> DPTYADYFSAWDKWEKQALPGEERDEAVSRLKECLINNSDELRLDRLNLSSLPDNLPAQITLLNVSYNQLTNLPELPVTLKKLYSASNKLSELPVLPPALESLQVQHNELENLPALPDSLLTMNISYNEIVSLPSLPQALKNLRATRNFLTELPAFSEGNNPVVREYFFDRNQISHIPESILNLRNECSIHISDNPLSSHALQALQRLTSSPDYHGPRIYFSMSDGQQNTLHRPLADAVTAWFPENKQSDVSQIWHAFEHEEHANTFSAFLDRLSDTVSARNTSGFREQVAAWLEKLSASAELRQQSFAVAADATESCEDRVALTWNNLRKTLLVHQASEGLFDNDTGALLSLG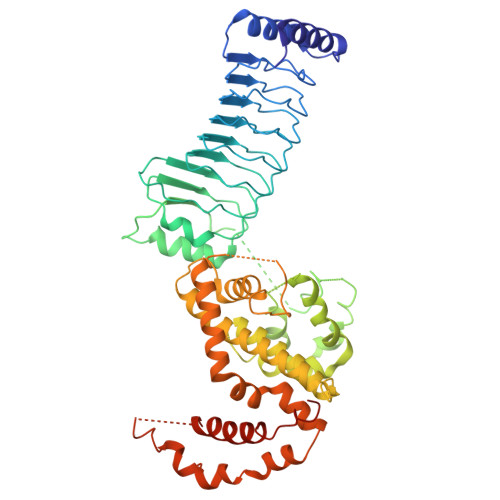REMFRLEILEDIARDKVRTLHFVDEIEVYLAFQTMLAEKLQLSTAVKEMRFYGVSGVTANDLRTAEAMVRSREENEFTDWFSLWGPWHAVLKRTEADRWAQAEEQKYEMLENEYPQRVADRLKASGLSGDADAEREAGAQVMRETEQQIYRQLTDEVLALRLSENGSQLHHS> MEDLNFEERGSTQIPASLQQHFSAKLGRQNELEKTPSRGGLGLV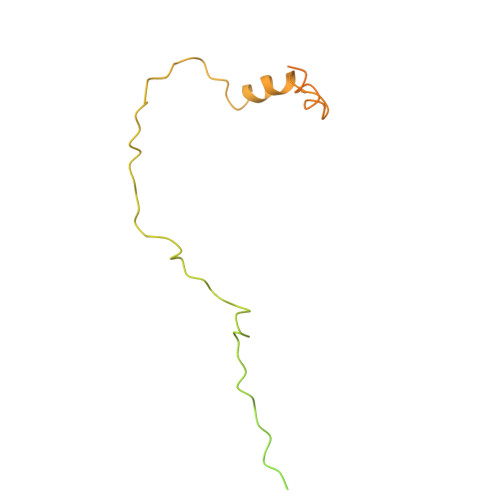VNSSKTPGGKSLQSLASACKVPPSTKKNTIPIAFECYEDETDDQIADVATIKKTEKHPCSPIDTANRCETFDSLAADIEDDMLNLEDQDVVLSEDRPYGDVIDPAESEAEALAELGVEEWDSYPPIDPASRIGDDFNYVLRTEDFAEEGDVKLEETRHRTVIADIDEVKMSKAERNELFSMLADDLDSYDLLAEEANLPL[(1S)-2-(methoxycarbonylamino)-1-phenyl-ethoxy]-propyl-phosphinic 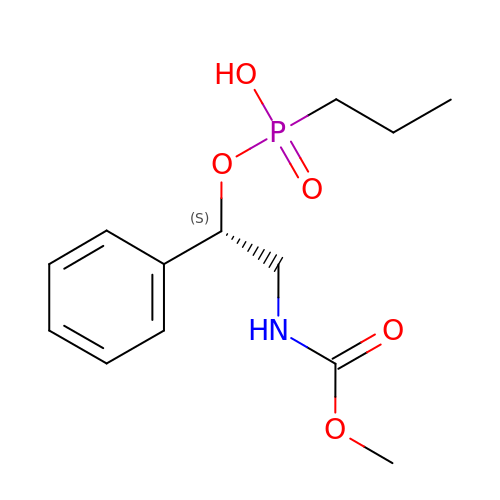acid | C13 H20 N O5 P | LJRNVQUHAPUUFK-GFCCVEGCSA-N> MEIDELTALGGLLHDIGKPVQRAGLYSGDHSTQGARFLRDLAENTGRAEYELLSLFSEFHHKGHMKNDELMIRRIKELSPERFGLTMEDVLNALWIVYEADNLASGEREEGQPQASRPLYSVFNPGKAYPWAELDFEKELPVPGDVFSIRSQDYRELVKRLWEELSKAKLRSDRLLPVLEKYLTFVSSVTSEGNIISLYDHMRMTSAIALAMLRAGCTAEDVRSGRCRKEKRFLLIEGDFSGIQDFIYRVSGKGTLKYLRARSAYLELIGWDVVLEILSRLGLTRANVVFNAGGHFMIIAQNTPDAVKELEEIRAKAVEWLYREFESDLYLAIEWEPVSGREFGREGGKNLFAEARKRLKHKLTVRKLKRFGEIKGLFEHGHTERLAECPVCGRELPEGKLEPSASDPETKVCPTCNRLVSLGGNLPKLLGFGRTAKNDAGVLVEGPFSGFVPYLQGGRPVGEQILVKNTLNPGEIPESAQF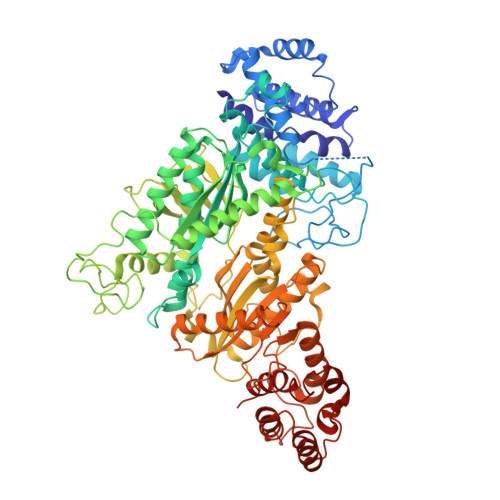VPYFVADYFKKDPKGGVATFEELSMASTGTRRLGVMKGDVDRLGEFFSSMDSPSKLATASRFMDYFFKGYIGAIIEGKFGYIIGDVPSLRDWPEEPDIVVVYAGGDDFFIVGAWDQIFELAFRVRRAFNAYTGGKLTLSVGLGYFDERTPIYRMADVVSERLDTAKDEGRNRVFVVGRSRPLDGKHKLSYEWNHYEELWRTYAPRIYAGNGRLKGKLESKKGLLWKLLEIRELYVRDPNDVRWAYLTAYLLGRHGLSDLFPELVGIDTKAVERKEPQPVYWVDGVLKIVLMAVRR>[6x]MTSAEMTSPNNNSEHQAIAKMRTMIEGFDDISHGGLPIGRSTLVSGTSGTGKTLFSIQFLYNGIIEFDEPGVFVTFEETPQ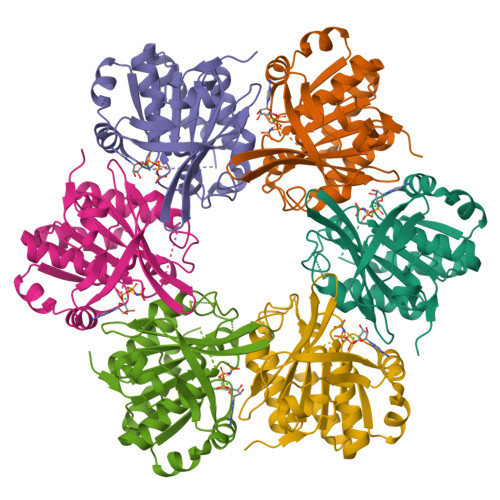DIIKNARSFGWDLAKLVDEGKLFILDASPDPEGQEVVGGFDLSALIERINYAIQKYRARRVSIDSVTSVFQQYDASSVVRRELFRLVARLKQIGATTVMTTERIEEYGPIARYGVEEFVSDNVVILRNVLEGERRRRTLEILKLRGTWHMKGEYPFTITDHGINIFPLGAMRL> MVIQVFRLNFRLRTGFRVGGGQEVGDNVIRQLRIGVEGVMIPASSWKGMFRRVSEIVLNSEDHFEEHSKKEVDTRTINALLKSDEKFRRIAISKVGKEVITQNGINVDKLDSESLSDLRRIYNEYNCPIERLYGSNYFAGGITI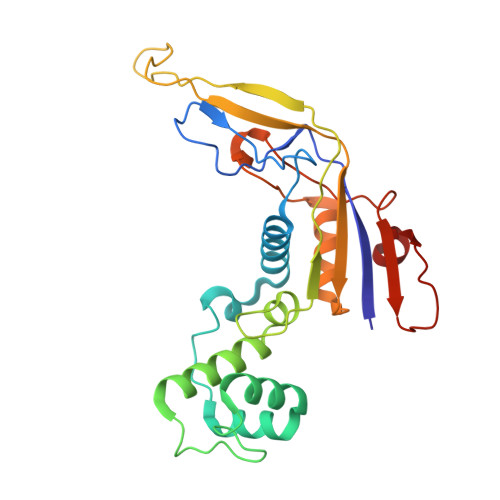SDSVIPNASIMERTHVTIERKSKKASEKHLFSEEIIDAEKIEVKVIVRNEFELWKNSLKLLREIGYFIGGSKSRGIGYIVLDEKESEYAVINNFSETPKFSELKRYLS> MIVSFMVAMDENRVIGKDNNLPWRLPSELQYVKKTTMGHPLIMGRKNYEAIGRPLPGRRNIIVTRNEGYHVEGCEVAHSVEEVFELCKNEEEIFIFGGAQIYDLFLPYVDKLYITKIHHAFEGDTFFPEMDMTNWKEVFVEKGLTDEKNPYT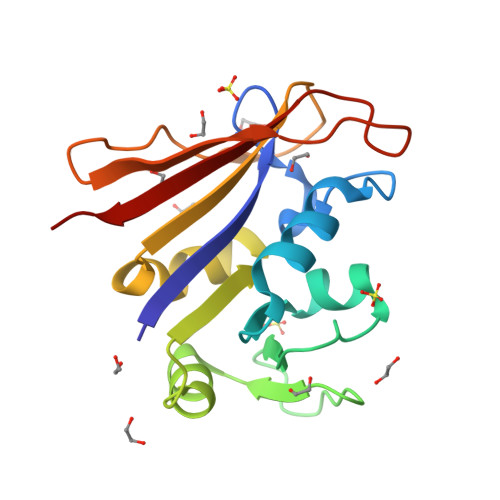YYYHVYEKQQ> KENEPPIRL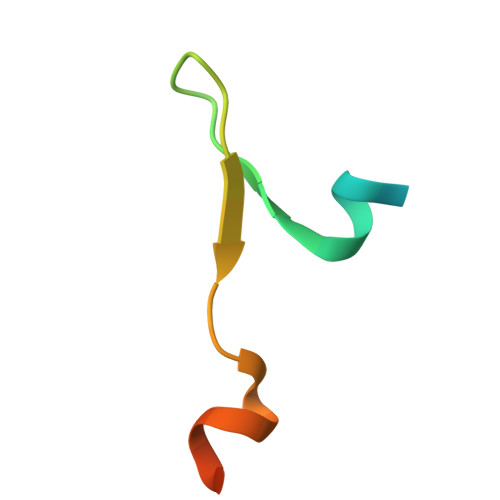LDDLFRKTKGTPCIYWLPLTPEAIAEKEAFR> MASIIAAKAKDKQYEIVGKAQNLLKQVQPLYNVGFSTTALDLLNAYFTYMQAQG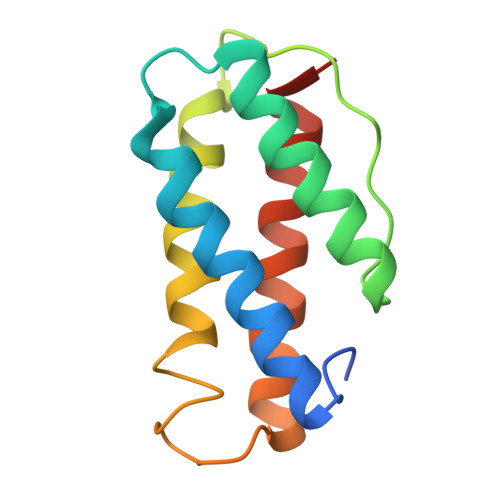FATTRAGTGFVSDGAKLARLDNMLDQVSKTGYVVLTGTGAPIGETSGTAFDTSFTALRAAFLAATTPTTA>[6x]IKLTKIKLDLPINFGPAFEGESIRKGDMYV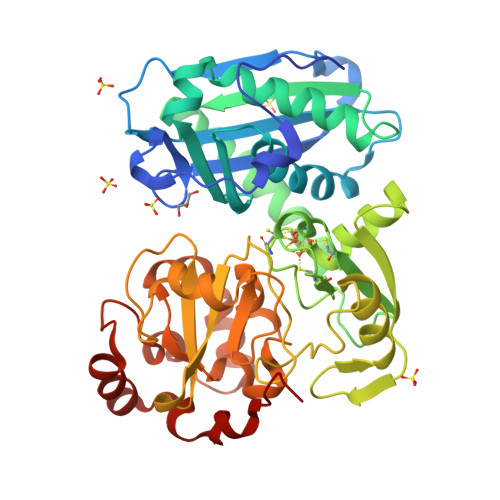EMGGNRTPAFELVRTVSESEITDGKIEVIGPDIDQIPEGSKLPLGILVDIYGRKMQADFEGVLERRIHDFINYGEGLWHTGQRNINWLRVSKDAVAKGFRFKNYGEILVAKMKEEFPAIVDRVQVTIFTDEAKVKEYMEVAREKYKERDDRMRGLTDETVDTFYSCVLCQSFAPNHVCIVTPERVGLCGAVSWLDAKASYEINHAGPNQPIPKEGEIDPIKGIWKSVNDYLYTASNRNLEQVCLYTLMENPMTSCGCFEAIMAILPECNGIMITTRDHAGMTPSGMTFSTLAGMIGGGTQTPGFMGIGRTYIVSKKFISADGGIARIVWMPKSLKDFLHDEVVRRSVEEGLGEDFIDKIADETIGTTVDEILPYLEEKGHPALTMDPIMRSHTSRGH> MARIRHVQGDITEFQGDAIVNAANNYLKLGAGVAGAILRKGGPSIQEECDRIGKIRVGEAAVTGAGN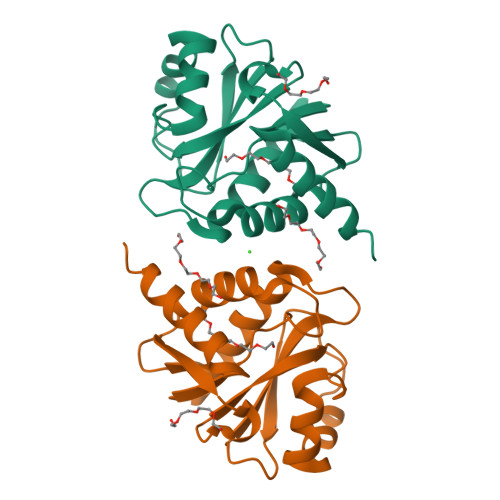LPVRYVIHAAVLGDEPASLETVRKATKSALEKAVELGLKTVAFTALGAWVGGLPAEAVLRVMLEEIKKAPDTLEVTGVHGTEKSAEAARRALLEHHHHHH>[2x]AEKTTRVGVNANLRSEQPVAAAVSYKVGTAGSPSKTNV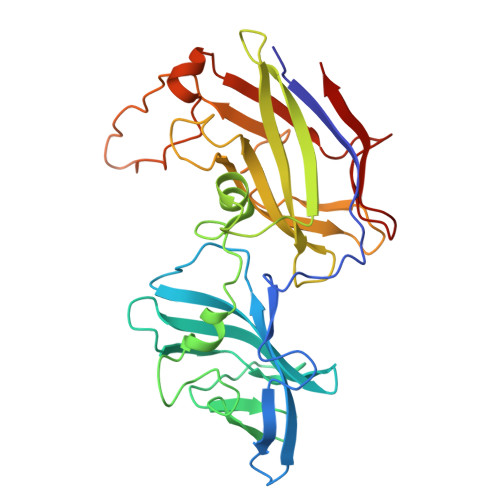VDSATNSHNYDVVYSSTGIANPVSGNNEYLVDIKENGVIVATGKVAYDAATNELVSSTIDYKGASPVTGSMTTTRINAAGTTVNLADLGIVNASGADDAEVVAGKLYDPSTWSMSDYAKDNSKGVKPDFEVQIPLSDSKGGQRTVTLSMLKGPGPNQWYAELRAKPGDLANNGNGQISTGIIEFTTDGKLKNTGSLFGTTSPTAITIKSSGYIAPTVTPPAVQPPTPPTWADALGIDEQEVQIDLASAAGGLTQYNSQSVVQSVNTNG>MPINKLRKRLGDLLVEEGIVSEAQLEQALNAQKNTGRRLGDTLISLGFLSETQLLNFLAQQLSLPVIDLSRAHVDIDAVPLLPEVHARRLRALVIGRSGDTLRIAMSDPADLFAQEALLNQLPDYGFEFVIAPEKQLVDGFDRYY[2x]

Recently, MshE (locus tag VC0405), an ATPase associated with the mannose-sensitive haemagglutinin type IV pilus (T4P) formation in Vibrio cholerae, as well as its homologue PA14_29490, an ATPase involved in the bacterial type II secretion system (T2SS) in Pseudomonas aeruginosa, were shown to be potent c-di-GMP-binding proteins. In both proteins, c-di-GMP binding has been localized to their N-terminal T2SSE_N (hereafter, MshEN) domains, whereas their C-terminal ATPase domains were shown to bind ATP but not c-di-GMP5. To explore the possibility that MshE contains a special kind of c-di-GMP-binding motif, we have solved the crystal structure of its MshEN domain (VcMshEN) in complex with c-di-GMP to a nearly-atomic level resolution of 1.37 Å. The structure revealed two 24-residue motifs linked together by 5 non-conserved residues that work cooperatively to form a 53-residue domain that binds a complete c-di-GMP molecule.

The VcMshEN structure was well-refined, and its macromolecular chain could be traced from residue Lys5 to Tyr145 without any interruption. Each MshEN structure could be further divided into two subdomains, a four-helix MshEN_N (α1−α4) and an α/β MshEN_C (a β1−β3 antiparallel β-sheet surrounded by three helices). C-di-GMP was bound mainly in the MshEN_N subdomain, with the only contribution from the MshEN_C subdomain coming from Asp108, which interacts with the amino group of the second guanine (Gua2) base of c-di-GMP. In VcMshEN, the N-terminal α1 helix is broken since the full α1 helix causes significant steric clash against c-di-GMP (cyan arrow). In addition, α2 helix in VcMshEN is extended by two turns and swings downward to enhance interaction with c-di-GMP (blue arrow). The first guanine base (Gua1) of c-di-GMP is stacked by the side chain atoms of Arg9 on one side, and by the hydrophobic residues Leu25, Leu29 and Leu39 on the other side, being sandwiched between the two hydrophobic surfaces. The backbone amide protons of the third Gly residue and the following non-conserved residue in the motif form two hydrogen bonds (H-bonds) with the O6 and N7 atoms of Gua1 via its Hoogsteen edge. Each of the two conserved Gln residues (Gln32 and Gln61) in the motif forms two H-bonds with the ribose 3'-OH and phosphate oxygen atom. Therefore the unique interactions of c-di-GMP with MshEN seem to be driven mainly by the three highly conserved hydrophobic Leu residues that form a triangular cluster to hold each guanine base via extensive CH-π bond interactions.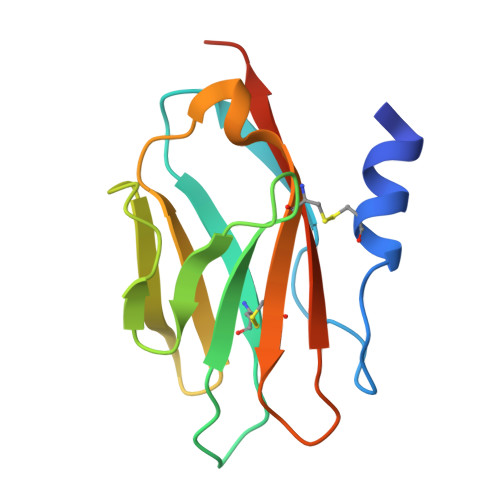> ADPASEEVMACLRQERSRVENPSQTIVNVVAENPAYLHCSVPPDAEHEIAWTRVSDGALLTAGNRTFTRDPRWQVSKKSANIWVLNLRRAEQQDSGCYLCEINDKHNTVYAVYLKVLEPHHHHHH>[44x]MYTNSDFVVIKALEDGVNVIGLTRGADTRFHHSEK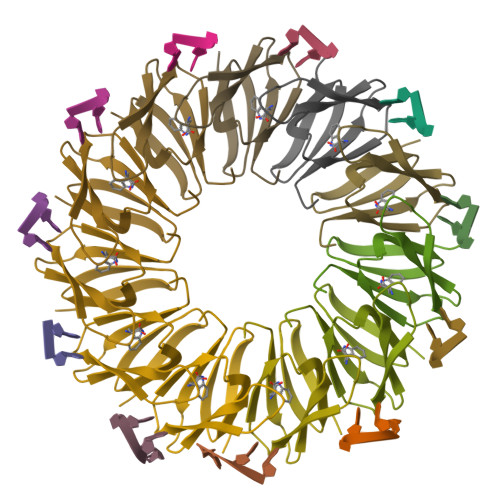LDKGEVLIAQFTEHTSAIKVRGKAYIQTRHGVIESEGKK> ARTXQTARKSTGG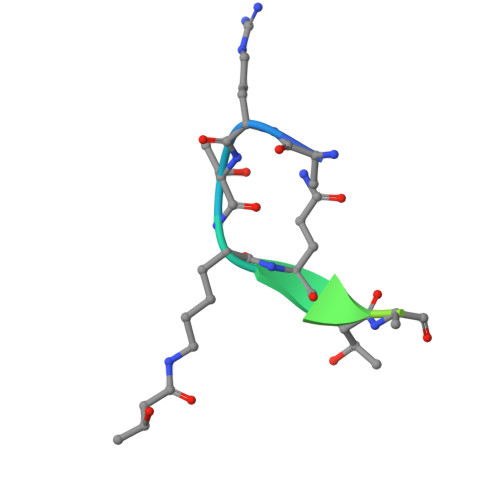KA>[2x]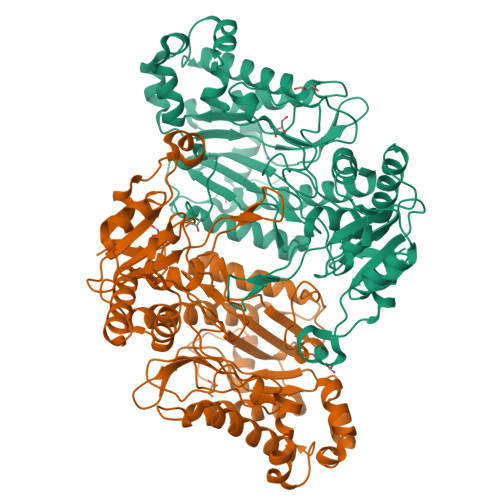MAAATGPSFWLGNETLKVPLALFALNRQRLCERLRKNPAVQAGSIVVLQGGEETQRYCTDTGVLFRQESFFHWAFGVTEPGCYGVIDVDTGKSTLFVPRLPASHATWMGKIHSKEHFKEKYAVDDVQYVDEIASVLTSQKPSVLLTLRGVNTDSGSVCREASFDGISKFEVNNTILHPEIVECRVFKTDMELEVLRYTNKISSEAHREVMKAVKVGMKEYELESLFEHYCYSRGGMRHSSYTCICGSGENSAVLHYGHAGAPNDRTIQNGDMCLFDMGGEYYCFASDITCSFPANGKFTADQKAVYEAVLRSSRAVMGAMKPGVWWPDMHRLADRIHLEELAHMGILSGSVDAMVQAHLGAVFMPHGLGHFLGIDVHDVGGYPEGVERIDEPGLRSLRTARHLQPGMVLTVEPGIYFIDHLLDEALADPARASFLNREVLQRFRGFGGVRIEEDVVVTDSGIELLTCVPHTVEEIEACMAGCDKAFTPFSGPK>[8x]MRGSHHHHHHGSMSELITE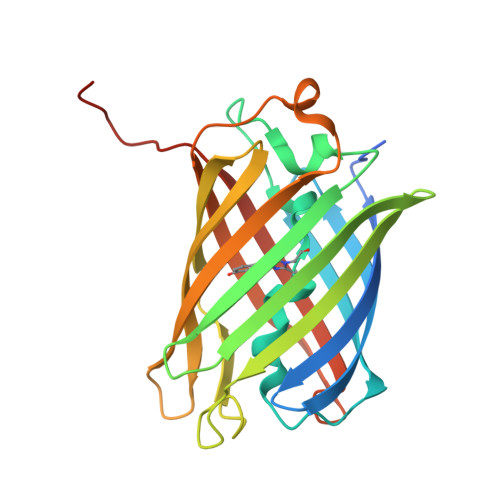NMHMKLYMEGTVNNHHFKCTSEGEGKPYEGTQTMRIKVVEGGPLPFAFDILATSFMYGSKTFINHTQGIPDFFKQSFPEGFTWERVTTYEDGGVLTATQDTSLQDGCLIYNVKIRGVNFPSNGPVMQKKTLGWEASTEMLYPADGGLEGRSDMALKLVGGGHLICNLKTTYRSKKPAKNLKMPGVYYVDRRLERIKEADKETYVEQHEVAVARYCDLPSKLGHKLN> MGSSHHHHHHSQDPMLEAKFEEASLFKRIIDGFKDCVQLVNFQCKEDGIIAQAVDDSRVLLVSLEIGVEAFQEYRCDHPVTLGMDLTSLSKILRCGNNTDTLTLIADNTPDSIILLFEDTKKDRIAEYSLKLMDIDADFLKIEELQYDSTLSLPSSEFSKIVRDLSQLSDSINIMITKETIKFVADGDIGSGSVIIKP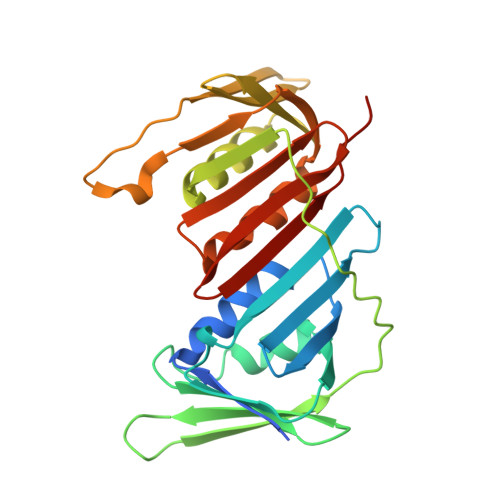FVDMEHPETSIKLEMDQPVDLTFGAKYLLDIIKGSSLSDRVGIRLSSEAPALFQFDLKSGFLQFFLAPKFNDEE> SMNPIEDELVFRVGSRGREKGEFTNLQGVSAASSGRIVVADSNNQCIQVFSNEGQFKFRFGVRGRSPGQLQRPTGVAVDTNGDIIVADYDNRWVSIFSPEGKFKTKIGAGRLMGPKGVAVDRNGHIIVVDNKSCCVFTFQPNGKLVGRFGGRGATDRHFAGPHFVAVNNKNEIVVTDFHNHSVKVYSADGEFLFKFGSHGEGNGQFNAPTGVAVDSNGNIIVADWGNSRIQVFDSSGSFLSYINTSAEPLYGPQGLALTSDGHVVVADAGNHCFKAYRYLQ

Tripartite motif (TRIM) proteins constitute one of the largest subfamilies of the RING-type E3 ubiquitin ligases that play a role in diverse processes from homeostasis and immune response to viral restriction. The NHL domain, or so-called NHL repeats named after ncl-1, HT2A and lin-41, forms another protein module found in four TRIMs, including TRIM2, TRIM3, TRIM32 and TRIM71, that constitute the subclass VII. Here, high-resolution crystal structures of the NHL domains of three of the four human TRIM–NHL proteins, namely TRIM2, TRIM3 and TRIM71, are presented. Comparative structural analyses revealed that, despite sharing an evolutionarily conserved six-bladed β-propeller architecture, the low sequence identities resulted in distinct properties of these interaction domains at their putative binding sites for macromolecules.

The NHL domains of TRIM2 and TRIM3 were highly expressed as a fusion protein with an N-terminal His6-GST tag in E. coli. Crystals of TRIM2 NHL were obtained within 1–2 d, while TRIM3 crystals grew within one week and TRIM71 crystals formed after approximately one month. The TRIM3 NHL structure was determined at 1.7 Å resolution from the tetragonal crystals that contained a single molecule in the asymmetric unit, whereas the monoclinic crystals of TRIM71 NHL diffracted to 2.2 Å resolution had an asymmetric unit consisting of two protein molecules. Nonetheless, an exception was noted when comparing TRIM2 and TRIM3 that were most similar with ∼82% sequence identity. In contrast, the rather shallow flat surface of the TRIM2/3 NHLs resembles that of their homologue DmBrat, which has been shown to recognize a linear RNA. However, comparative analyses suggest that similar binding of an RNA observed previously in DmBrat would be unlikely in TRIM2/3 due to the lack of a central channel as well as low sequence conservation within the pockets.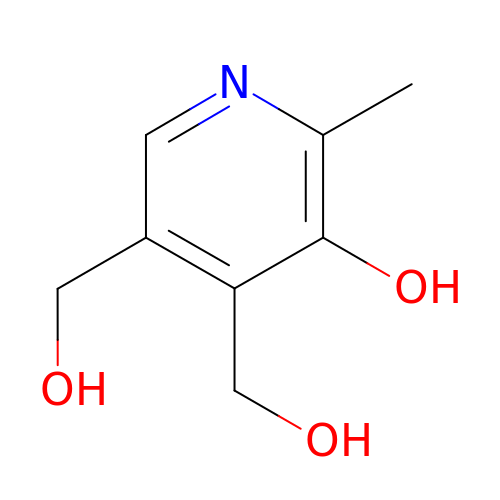4,5-bis(hydroxymethyl)-2-methyl-pyridin-3-ol | C8 H11 N O3 | LXNHXLLTXMVWPM-UHFFFAOYSA-N> MMSPNGSLKFASQAVAKPYFVFALILFVGQILFGLIMGLQYVVGDFLFPAIPFNVARMVHTNLLIVWLLFGFMGAAYYLVPEESDCELYSPKLAWILFWVFAAAGVLTILGYLLVPYAGLARLTGNELWPTMGREFLEQPTISKAGIVIVALGFLFNVGMTVLRGRKTAISMVLMTGLIGLALLFLFSFYNPENLTRDKFYWWWVVHLWVEGVWELIMGAILAFVLVKITGVDREVIEKWLYVIIAMALISGIIGTGHHYFWIGVPGYWLWLGSVFSALEPLPFFAMVLFAFNTINRRRRDYPNRAVALWAMGTTVMAFLGAGVWGFMHTLAPVNYYTHGTQ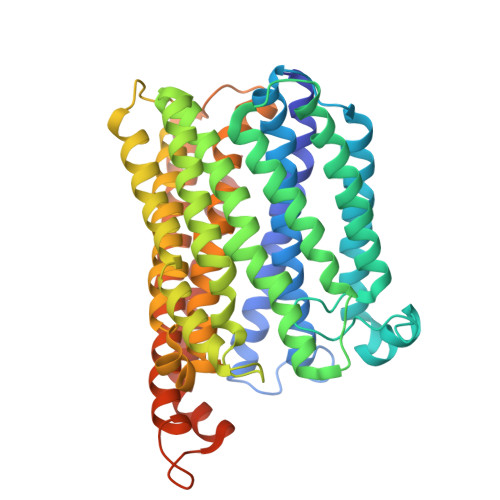LTAAHGHMAFYGAYAMIVMTIISYAMPRLRGIGEAMDNRSQVLEMWGFWLMTVAMVFITLFLSAAGVLQVWLQRMPADGAAMTFMATQDQLAIFYWLREGAGVVFLIGLVAYLLSFRRGKAAA> SLSCRPPMVKLVCPADNLRAEGLECTKTCQNYDLECMSMGCVSGCLCPPGMVRHENRCVALERCPCFHQGKEYAPGETVKIGCNTCVCQDRKWNCTDHVCDATCSTIGMAHYLTFDGLKYLFPGECQYVLVQDYCGSNPGTFRILVGNKGCSHPSVKCKKRVTILVEGGEIELFDGEVNVKRPMKDETHFEVVESGRYIILLLGKALSVVWDRHLSISVVLKQTYQEKVCGLCGNFDGIQNNDLTSSNLQVEEDPVDFGNSWKVSSQCADTRKVPLDSSPATCHNNIMKQTMVDSSCRILTSDVFQDCNKLVDPEPYLDVCIYDTCSCESIGDCACFCDTIAAYAHVCAQHGKVVTWRTATLCPQSCEERNLRENGYECEWRYNSCAPACQVTCQHPEPLACPVQCVEGCHAHCPPGKILDELLQTCVDPEDCPVCEVAGRRFASGKKVTLNPSDPEHCQICHCDVVNLTCEACQEPGGLVV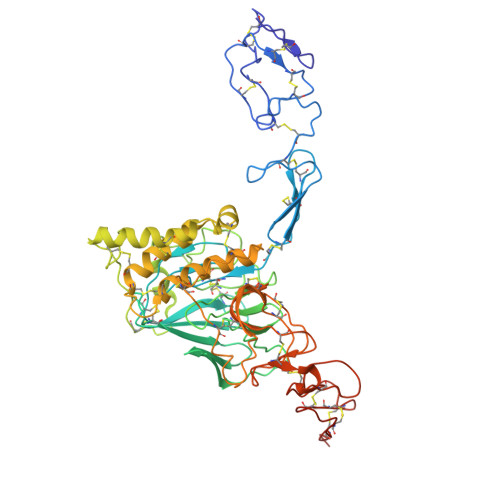PPHHHHHH>MTELSPTALDPTELRSSLDKPFGTNRVIADDAMMADSITPAQYRYHHGSRVRPVNWNNIVDDKDLDVWNRLIANFWLPEKVPLSNDIPSWRSLTDLERKTTTRVFTGLTLLDTSQATIGELCQIEHARTEHEQAIYTNIAFMQSIHARSYSSIFSTLCSSEEIDEAYRWAVGNDVLQQRVTTVLCEYESEDPLKRKIAATMLSSLLLYAGFYLPLYFASRGKMMNTADMIRLILRDKAIHGYYSGYKFQRGLELRSENDKKNLEKF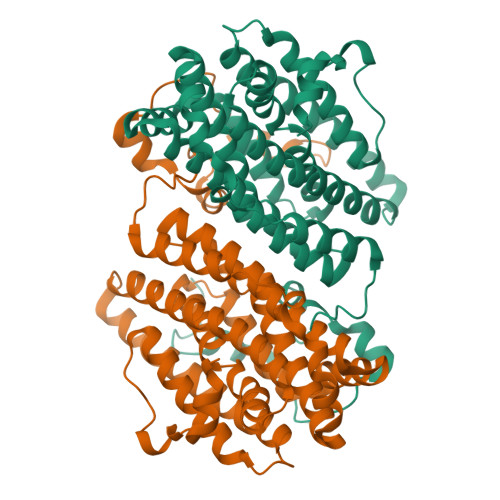TMNLLDTLYDLEVEYSGQIYEGFDFHDDVFDFVRYNANKALMNLGYPAKYSEEETHVSPEILAALSPAADENHDFFSGSGSSYIMGKSVETDDDDWDF[4x]7-methyl-2H-1,4-benzothiazin-3(4H)-one | C9 H9 N O S | 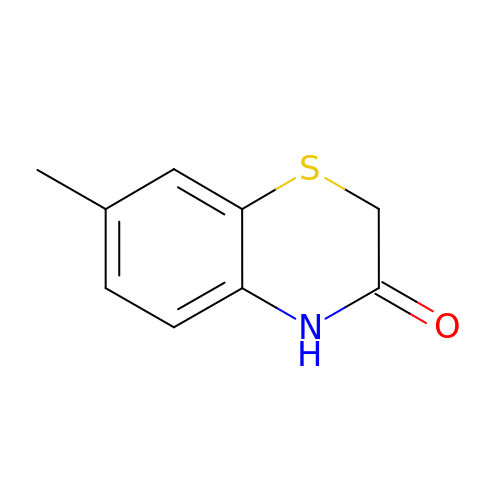ODJQMWDFNLNCTM-UHFFFAOYSA-N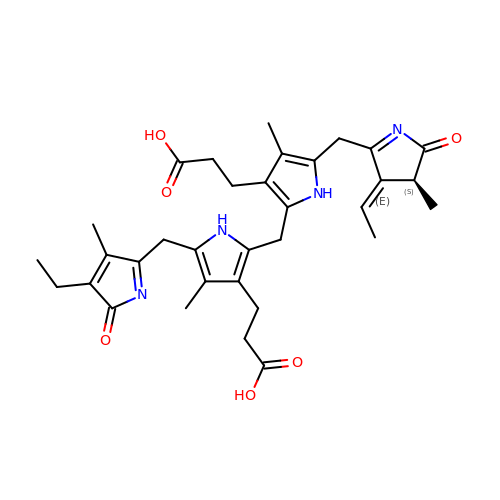3-[2-[[5-[[(3E,4S)-3-ethylidene-4-methyl-5-oxidanylidene-pyrrol-2-yl]methyl]-3-(3-hydroxy-3-oxopropyl)-4-methyl-1H-pyrrol-2-yl]methyl]-5-[(4-ethyl-3-methyl-5-oxidanylidene-pyrrol-2-yl)methyl]-4-methyl-1H-pyrrol-3-yl]propanoic acid | C33 H40 N4 O6 | YHFJLIYOVARRSS-AYZAYIPBSA-N>XGEI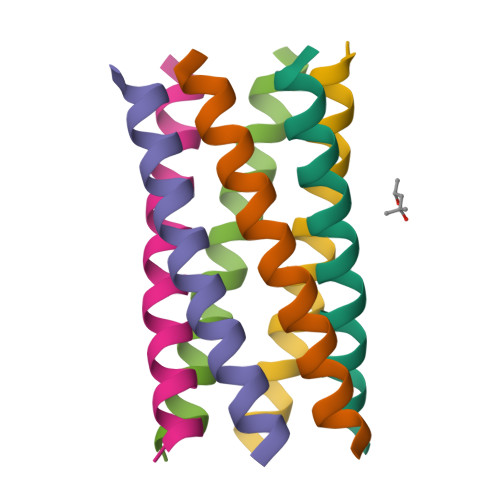AQALKEIAKAAKEIAWALKEIAQALKGX[6x]>[4x]MDMYTAIVNLKTYREATGANFTRFMEKFEPVQGKFELIFSPSLLDLEKAAKCGKFRFFAQHVDAEPYGAYTGHV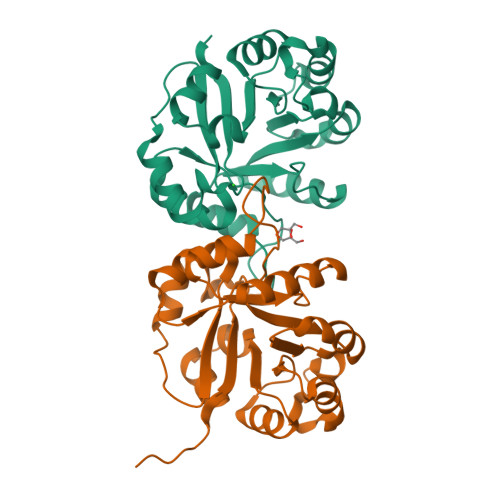PMDMMIDLGITGSILNHSERRLPRDTIINTLKKASKLDFTIVLCVENAEEAKYFREYEPDFIAYEPRDLIGGDVSVSTAKPEIIEDIVKIYEGTGTSVLVGAGIKTGEDVRRSIGLGARGILVASGVVKSADPTKSLNSLIELKLEHHHHHH>DSFLQRYSSDPTG[2x];>[2x]GSLIGLMKDAFQPHHHHHHHLSPHPPGTVDKKMVEKCWKLMDKVVRLCQNPKLALKNSPPYILDLLPDTYQHLRTILSRYEGKMETLGENEYF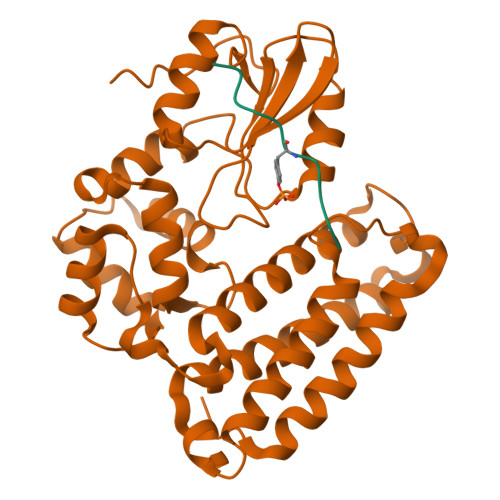RVFMENLMKKTKQTISLFKEGKERMYEENSQPRRNLTKLSLIFSHMLAELKGIFPSGLFQGDTFRITKADAAEFWRKAFGEKTIVPWKSFRQALHEVHPISSGLEAMALKSTIDLTCNDYISVFEFDIFTRLFQPWSSLLRNWNSLAVTHPGYMAFLTYDEVKARLQKFIHKPGSYIFRLSCTRLGQWAIGYVTADGNILQTIPHNKPLFQALIDGFREGFYLFPDGRNQNPDLTG>MAPVLSKDVADIESILALNPRTQSHAALHSTLAKKLDKKHWKRNPDKNCFHCEKLENNFDDIKHTTLGERGALREAMRCLKCADAPCQKSCPTHLDIKSFITSISNKNYYGAAKMIFSDNPLGLTCGMVCPTSDLCVGGCNLYATEEGSINIGGLQQFASEVFKAMNIPQIRNPCLPSQEKMPEAYSAKIALLGAGPASISCASFLARLGYSDITIFEKQEYVGGLSTSEIPQFRLPYDVVNFEIELMKDLGVKIICGKSLSENEITLNTLKEEGYKAAFIGIGLPEPKTDDIFQGLTQDQGFYTSKDFLPLVAKSSKAGMCACHSPLPSIRGAVIVLGAGDTAFDCATSALRCGARRVFLVFRKGFVNIRAVPEEVELAKEEKCEFLPFLSPRKVIVKGGRIVAVQFVRTEQDETGKWNEDEDQIVHLKADVVISAFGSVLRDPKVKEALSPIKFNRWDLPEVDPETMQTSEPWVFAGGDIVGMANTTVESVNDGKQASWYIHKYIQAQYGASVSAKPELPLFYTPVDLVDISVEMAGLKFINPFGLASAAPTTSSSMIRRAFEAGWGFALTKTFSLDKDIVTNVSPRIVRGTTSGPMYGPGQSSFLNIELISEKTAAYWCQSVTELKADFPDNIVIASIMCSYNKNDWMELSRKAEASGADALELNLSCPHGMGERGMGLACGQDPELVRNICRWVRQAVQIPFF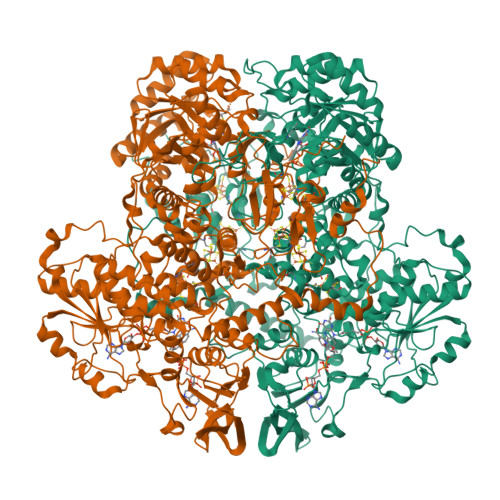AKLTPNVTDIVSIARAAKEGGADGVTATNTVSGLMGLKADGTPWPAVGAGKRTTYGGVSGTAIRPIALRAVTTIARALPGFPILATGGIDSAESGLQFLHSGASVLQVCSAVQNQDFTVIQDYCTGLKALLYLKSIEELQGWDGQSPGTESHQKGKPVPRIAELMGKKLPNFGPYLEQRKKIIAEEKMRLKEQNAAFPPLERKPFIPKKPIPAIKDVIGKALQYLGTFGELSNIEQVVAVIDEEMCINCGKCYMTCNDSGYQAIQFDPETHLPTVTDTCTGCTLCLSVCPIIDCIRMVSRTTPYEPKRGLPLAVNPVC[4x]N1-[(1R)-1-(DIHYDROXYBORYL)ETHYL]-N2-[(TERT-BUTOXYCARBONYL)-D-GAMMA-GLUTAMYL]-N6-[(BENZYLOXY)CARBONYL-L-LYSINAMIDE | C26 H41 B N4 O10 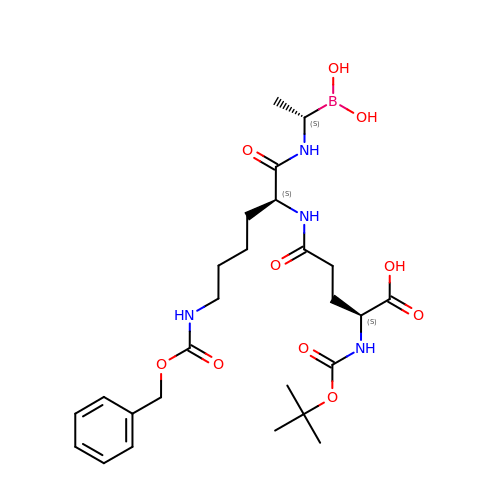| OTTYWVUOPWENAJ-HOJAQTOUSA-N>MAIKRGADLIVEALEEYGTEQVVGFIGHTSHFVADAFSKSHLGKRVINPATELGGAWMVNGYNYVKDRSAAVGAWHCVGNLLLHAAMQEARTGRIPAVHIGLNSDGRLAGRSEAAQQVPWQSFTPIARSTQRVERLDKVGEAIHEAFRVAEGHPAGPAYVDIPFDLTADQIDDKALVPRGATRAKSVLHAPNEDVREAAAQLVAAKNPVILAGGGVARSGGSEALLKLAEMVGVPVVTTSTGAGVFPETHALAMGSAGFCGWKSANDMMAAADFVLVLGSRLSDWGIAQGYITKMPKFVHVDTDPAVLGTFYFPLLSVVADAKTFMEQLIEVLPGTSGFKAVRYQERENFRQATEFRAAWDGWVREQESGDGMPASMFRAMAEVRKVQRPEDIIVTDIGNHTLPMFGGAILQRPRRLVTSMAEGILGCGFPMALGAQLAEPNSRVFLGTGDGALYYHFNEFRVAVEHKLPVITMVFTNESYGANWTLMNHQFGQNNWTE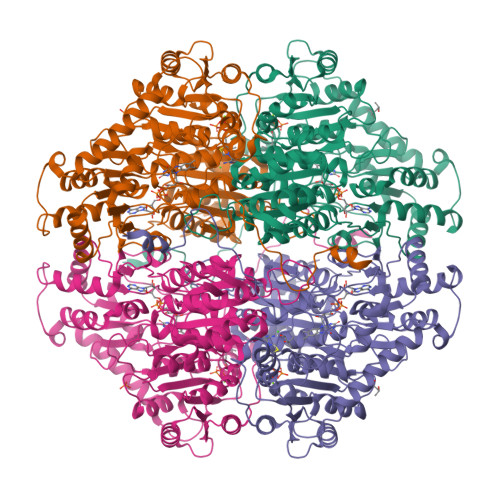FMNPDWVGIAKAFGAYGESVRETGDIAGALQRAIDSGKPALIEIPVSKTQGLASDPVGGVGPNLLLKGREIPVDTGGSMYPGENLLHLKS[2x]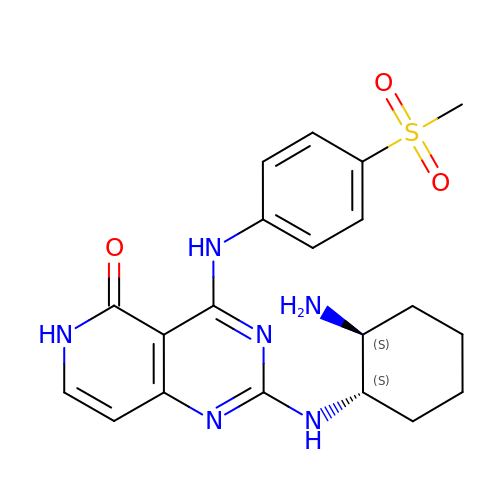2-[[(1S,2S)-2-azanylcyclohexyl]amino]-4-[(4-methylsulfonylphenyl)amino]-6H-pyrido[4,3-d]pyrimidin-5-one | C20 H24 N6 O3 S | DVWCWBAFIKQUNR-GJZGRUSLSA-N>[4x]GPLGSVREEIESLVQDSLMEMVKGVKNTIESDLASKKGLAQSTTEILQLDPTNKAFAKSVLESPNLKGSFLAIGLGYESDATVVENDDGWEPN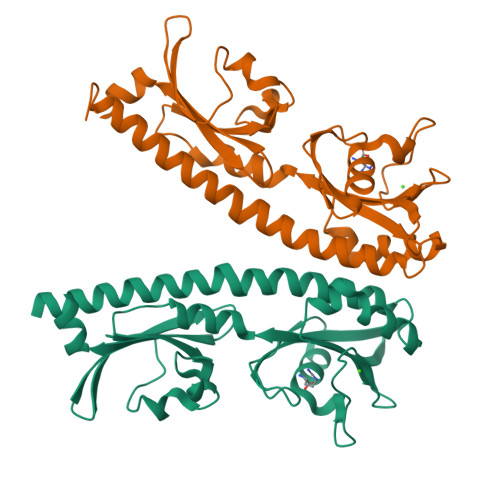ADYDPRKRPWYVDAKRERKLVVTEPYVDISTKKIIISIGTPVYQQSNFVGAMFYDVELTQLAQLVNSVNLFDAGYLFITTKDGVTIAHPNAENNGEKFSQFLPNVDLKEGTQRIELDGKYYLVKFAQVPSESWYIGAVVDESIAFAMVDDLRHSSLIHHHHHH> KPISPEQEELIHRLVYFQNEYEQPSDEDFRHITEITILTVQLIVEFAKRLPGFDKLLREDQIALLKACSSEVMMLRMARRYDVGSDSILATVDDLLRFCRQMYGMKVDNAEYALLTAIVIFSERPSLIEGWKVEKIQEIYLEALKVYVDNRRKPRSGTIFAKLLSVLTELRTLGNLNSEMCFSLKLKNKKLPPFLAE;> AANAVANICQATNTQLYQLVEWAKHIPHFSSLPIEDQVLLLRAGWNELLIAAFSHRSVEVRDGIVLGAGITVHRNSAHQAGVGTIFDRVLTELVAKMRDMNMDRTELGSLRSIILFNPEVRGLKSGQEVELLREKVYAALEEYTRVTRPEEPGRFAKLLLRLPALRSIGLKCLE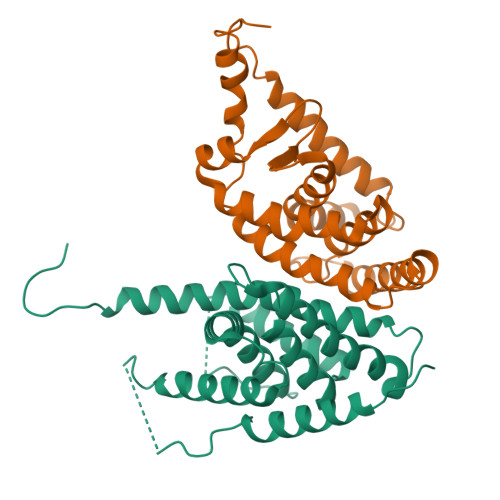HLFFFRLIGDIPIDTFLMDMLG>[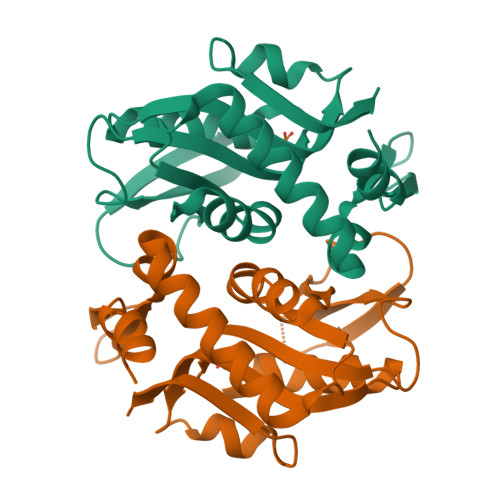2x]DSELQLVEQRIRSFPDFPTPGVVFRDISPVLKDPASFRAAIGLLARHLKATHGGRIDYIAGLDSRGFLFGPSLAQELGLGCVLIRKRGKLPGPTLWASYSLEYGKAELEIQKDALEPGQRVVVVDDLLATGGTMNAACELLGRLQAEVLECVSLVELTSLKGREKLAPVPFFSLLQYE> IVGGYTCGANTVPYQVSLNSGYHFCGGSLINSQWVVSAAHCYKSGIQVRLGEDNINVVEGNEQFISASKSIVHPSYNSNTLNNDIMLIKLKSAASLNSRVASISLPTSCASAGTQCLISGWGN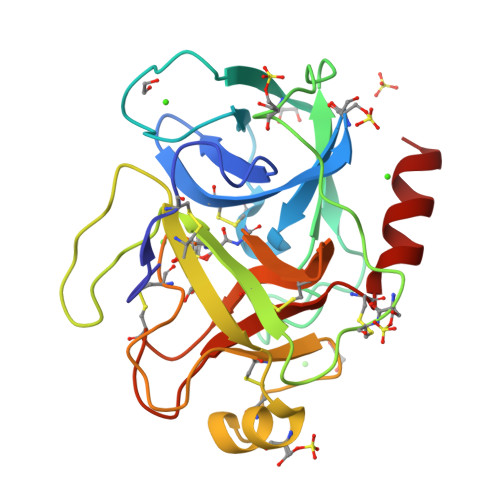TKSSGTSYPDVLKCLKAPILSDSSCKSAYPGQITSNMFCAGYLEGGKDSCQGDXGGPVVCSGKLQGIVSWGSGCAQKNKPGVYTKVCNYVSWIKQTIASN>MKRIGVLTSGGASPGMNAAIRSVVRKAIYHGVEVYGVYHGYAGLIAGNIKKLEVGDVGDIIHRGGTILYTARCPEFKTEEGQKKGIEQLKKHGIEGLVVIGGDGSYQGAKKLTEHGFPCVGVPGTIDNDIPGTDFTIGFDTALNTVIDAIDKIRDTATSHERTYVIEVMGRHAGDIALWSGLAGGAETILIPEADYDMNDVIARLKRGHERGKKHSIIIVAEGVGSGVDFGRQIQEATGFETRVTVLGHVQRGGSPTAFDRVLASRLGARAVELLLEGKGGRCVGIQNNQLVDHDIAEALANKHTIDQRMYA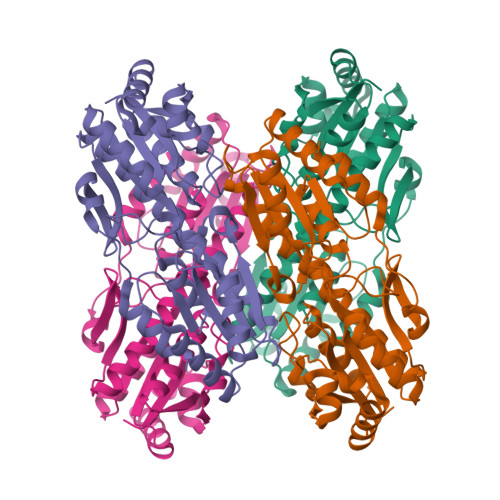LSKELSI[4x]>MTSCHIAEEHIQKVAIFGGTHGNELTGVFLVKHWLENGAEIQRTGLEVKPFITNPRAVKKCTRYIDCDLNRIFDLENLGKKMSEDLPYEVRRAQEINHLFGPKDSEDSYDIIFDLHNTTSNMGCTLILEDSRNNFLIQMFHYIKTSLAPLPCYVYLIEHPSLKYATTRSIAKYPVGIEVGPQPQGVLRADILDQMRKMIKHALDFIHHFNEGKEFPPCAIEVYKIIEKVDCPRDENGEIAAIIHPNLQDQDWKPLHPGDPMFLTLDGKTIPLGGDCTVYPVFVNEA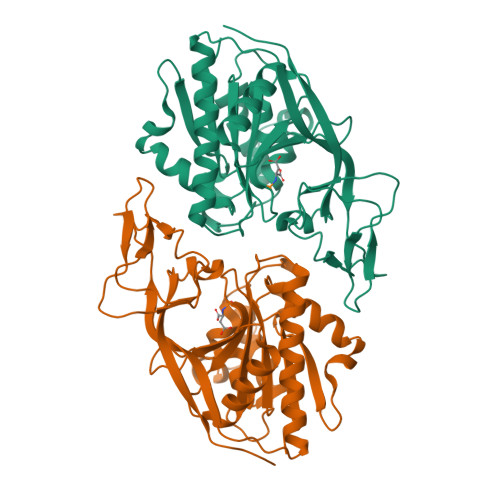AYYEKKEAFAKTTKLTLNAKSIRCCLH[2x]>MRGSPRTKDRLAALKAAVSDEEDVEEVAVQVDSGGGFMEEFFEQVEEIRAMIDKISDNVDAVKKKHSDILSAPQTDDQMKEELEELMTDIKRTANKVRGKLKTIELNIEQEEHSNKSSADLRIRKTQYSTISRKFVEVMSDYNTTQIDYRDRCKARIKRQMEITGRTTTNEELEDMLESG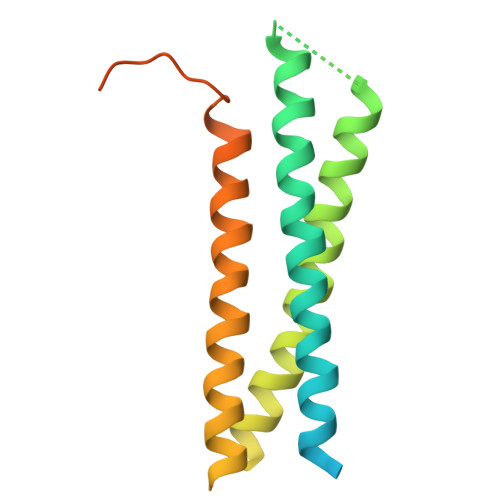[2x]> MAAQGFL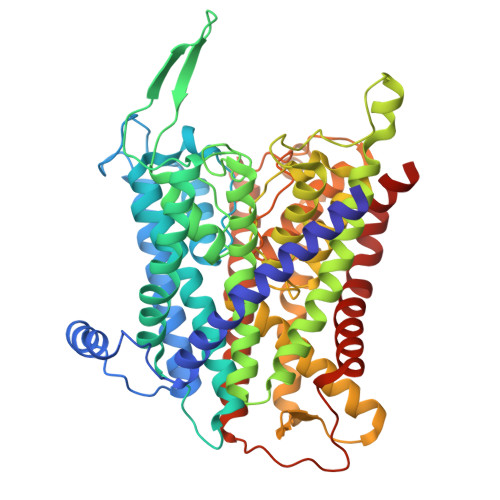LIATFLLVLMVLARPLGSGLARLINDIPLPGTTGVERVLFRALGVSDREMNWKQYLCAILGLNMLGLAVLFFMLLGQHYLPLNPQQLPGLSWDLALNTAVSFVTNTNWRSYSGETTLSYFSQMAGLTVQNFLSAASGIAVIFALIRAFTRQSMSTLGNAWVDLLRITLWVLVPVALLIALFFIQQGALQNFLPYQAVNTVEGAQQLLPMGPVASQEAIKMLGTNGGGFFNANSSHPFENPTALTNFVQMLAIFLIPTALCFAFGEVMGDRRQGRMLLWAMSVIFVICVGVVMWAEVQGNPHLLALGTDSSINMEGKESRFGVLVSSLFAVVTTAASCGAVIAMHDSFTALGGMVPMWLMQIGEVVFGGVGSGLYGMMLFVLLAVFIAGLMIGRTPEYLGKKIDVREMKLTALAILVTPTLVLMGAALAMMTDAGRSAMLNPGPHGFSEVLYAVSSAANNNGSAFAGLSANSPFWNCLLAFCMFVGRFGVIIPVMAIAGSLVSKKSQAASSGTLPTHGPLFVGLLIGTVLLVGALTFIPALALGPVAEYLS>SRPHQWQTDEEGVRTGKCSFPVKYLGHVEVDESRGMHICEDAVKRLKAERKFFKGFFGKTGKKAVKAVLWVSADGLRVVDEKTKDLIVDQTIEKVSFCAPDRNFDRAFSYICRDGTTRRWICHCFMAVKDTGERLSHAVGCAFAACLERKQKREKE[4x];>[4x]AYIGPYL

Numb functions as an oncosuppressor by inhibiting Notch signaling and stabilizing p53. Numb can also bind to Mdm2, thereby inhibiting its ubiquitin–ligase activity on p53, which physiologically destines the latter to proteasomal degradation. In the four isoforms of Numb, the PTB domain is present as a short version (PTBo in isoform 3 and 4) or a long one (PTBi in isoform 1 and 2), differing for the presence of a stretch of 11 aa coded by Ex3. In this study, we demonstrate that the sequence encoded by Ex3 (11 aa) is responsible for binding to Mdm2 and recapitulates the effects of holo-Numb on p53 and p53-dependent phenotypes.

We determined the crystallographic structure of Numb-PTBi bound to a phosphopeptide (GPpY) derived from a “canonical” PTB-binding adapter protein at 2.8 Å resolution. In the two crystal forms obtained, the canonical PTB fold was extended by the insertion of the Ex3-encoded sequence. The 11-residue Ex3 loop was found to adopt three conformations, all characterized by extension of helix α2 of one or two turns. The crystal structure of Numb-PTBi showed that the Ex3 sequence connects the α2 helix to the β2 strand of the PTBi module adopting several conformations without altering the hydrophobic core of the domain. Ex3 contributed to the formation of a large positively charged patch contributed by lysines 63, 66, 81, 82, and 85 and arginine 64 from Ex3 and flanking regions in the core PTB fold. In addition, the “canonical” phosphopeptide-binding region of the PTB domain was remote and completely distinct from the Ex3-coded region. Indeed, by a variety of approaches, we were able to show that the peptide-binding cleft of PTBi is not involved in the interaction with Mdm2.>GSHMASKGNIEVLNLVTGPDSITTIELYLNTRMGQNDESKDNYGYSEKVTVANSSDQDKPTSGEIPTYSTARINLPMLNEDLTCNTLTMWEAVSVKTEVVGVSSLVNVHMATKRMYDDKGIGFPVEGMNFHMFAVGGEPLELQFLTGNYRTDYSANDKLVVPPIKHQSTQGLNPHYKQKLTKDGAFPVECWCPDPSKNENTRYYGSYTGGQSTPPVLQFTNTVTTVLLDENGVGPLCKGDGLYVSCCDIVGFLVGKDGDMQYRGLPRYFNILLRKRTVRN[5x]

Trichodysplasia spinulosa-associated Polyomavirus (TSPyV) was isolated from a patient suffering from trichodysplasia spinulosa, a skin disease that can appear in severely immunocompromised patients. TSPyV has a 5232-nucleotide dsDNA genome encapsulated in its non-enveloped icosahedral capsid made up of the proteins VP1, VP2 and VP3. As is typical for polyomaviruses, the TSPyV VP1 monomer adopts the iconic jelly-roll fold with a conserved core comprising two β-sheets that are formed by strands B, I, D, G and C, H, E, F, respectively. We demonstrate here that the skin-tropic TSPyV binds sialylated glycans in a binding site formed by the BC2-loop on top of the VP1 protein that is not utilized by any other structurally characterized member of the polyomavirus family.

To establish a platform for understanding the specificity of the interaction with sialic acid, we solved crystal structures of TSPyV VP1 alone and in complex with three different sialylated compounds, the branched α2,3-linked GM1 pentasaccharide and the linear glycans α2,3- and α2,6-sialyllactose (3’SL and 6’SL, respectively). TSPyV VP1 pentamers were co-crystallized in the presence of either 10 mM GM1 glycan or 10 mM 6’SL, while preformed native TSPyV VP1 pentamer crystals were derivatized by soaking them in a 10 mM 3’SL solution for complex formation. The highest occupancy was obtained for GM1 in all five binding sites of the VP1 pentamer in the asymmetric unit, and so additional glycan residues besides Neu5Ac could be built unambiguously into well-defined electron density. Nevertheless, three of the five binding sites were not considered for further structural analysis because the ligand participates in crystal contacts. In the remaining two sites of the VP1 pentamer, the Neu5Ac residue and the GalNAcβ1-3(Neu5Acα2–3)Gal trisaccharide, respectively, are well-defined by electron density and distant from crystal contacts. The N-acetyl group of Neu5Ac inserts into a shallow cavity that is built by the BC2-loop on top of a VP1 monomer, thereby forming hydrogen bonds via its NH-group towards the hydroxyl side chain of threonine 73 and via its oxygen with the backbone amino group of lysine 82. The side chain of the arginine residue 137 from the DE-loop of the counterclockwise (ccw) VP1 monomer interacts with the glycerol chain of Neu5Ac. Residue H132 of the ccw monomer forms the bottom of the shallow binding groove so that the methyl group of Neu5Ac is recognized via hydrophobic interactions by the non-polar part of the ccw H132 side and by BC2-loop residues A75 and P83. The average B-factor of the Neu5Ac ring of GM1 is in the same range as those of the neighboring protein residues, indicating that the occupancy is near 1.0 for the ligand. We found that TSPyV VP1 interacts with the GM1 glycan in solution.>PPQKIEIFKSLDNWAEENILVHLKPVEKCWQPQDFLPDPASDGFDEQVRELRERAKEIPDDYFVVLVGDMIKEEALPTYQTMLNTLDGVRDETG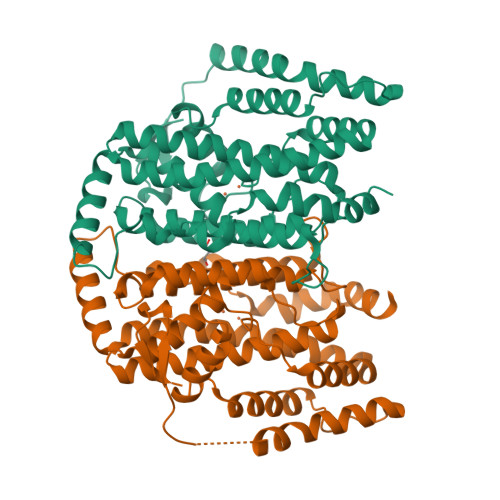ASPTSWAIWTRAWTAEENRHGDLLNKYLYLSGRVDMRQIEKTIQYLIGSGMDPRTENSPYLGFIYTSFQERATFIEHGNTARQAKEHGDIKLAQICGTIAADEKRHETAYTKIVEKLFEIDPDGTVLAFADMMRKKISMPAHLMYDGRDDNLFDHFSAVAQRLGVYTAKDYADILEFLVGRWKVDKLTGLSAEGQKAQDYVCRLPPRIRRLEERAQGRAKEAPTMPFSWIFDRQVKL[6x]> GLPTMNTPGSCQFLTSDDFQSPSAMPQYDVTPEMRIPGEVKNLMEIAEVDSVVPVQNVGEKVNSMEAYQIPVRSNEGSGTQVFGFPLQPGYSSVFSRTLLGEILNYYTHWSGSIKLTFMFCGSAMATGKFLLAYSPPGAGAPTKRVDAMLGTHVVWDVGLQSSCVLC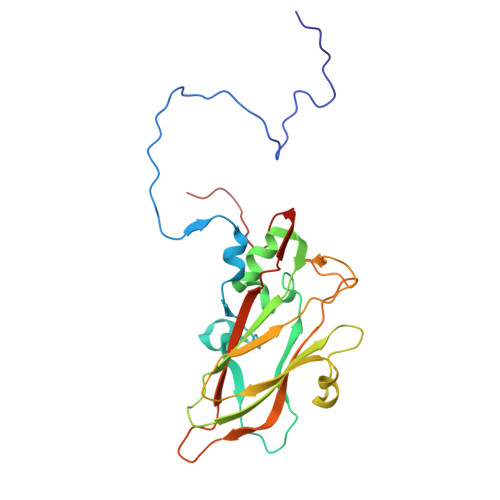IPWISQTHYRYVASDEYTAGGFITCWYQTNIVVPADAQSSCYIMCFVSACNDFSVRLLKDTPFISQENFFQ> NAKGNYCKRTPLYIDFKEIGWDSWIIAPPGYEAYECRGVCNYPLAEHLTPTKHAIIQALVHLKNSQKASKACCVPTKLEPISILYLDKGVVTYKFKYEGMAVSECGCR;> GSQNQERLCAFKDPYQQDLGIGESRISHENGTILCSKGSTCYGLWEKSKGDINLVKQGCWSHIGDPQECHYEECVVTTTPPSIQNGTYRFCCCSTDLCNVNFTENFPPPDT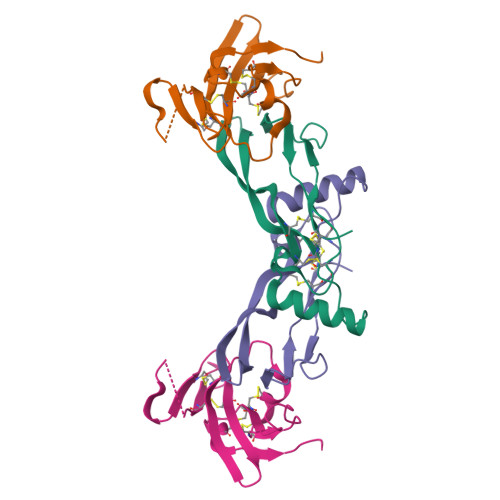TPLSPPHSFNRDET> GPMSQVLFHQLVPLQVKCKDCEERRVSIRMSIELQSVSNPVHRKDLVIRLTDDTDPFFLYNLVISEEDFQSLKFQQGLLVDFLAFPQKFIDLLQQCTQEHAKEIPRFLLQLVSPAAILDNSPAFLNVVETNPEKHLTHLSLKLLPGNDVEIKKF

Centriole assembly requires oligomerization of the essential protein spindle assembly abnormal 6 (SAS-6), which forms a structural scaffold templating the organization of further organelle components. SAS-6 is an essential protein for centriole formation and a key component of a scaffold-like structure known as the “cartwheel” or “central tube”. Crystallographic, EM, atomic force microscopy, and biophysical studies of SAS-6 variants from multiple species have shown that SAS-6 oligomerization is driven by two dimerization interfaces mediated by the protein “head” domain and a homodimeric coiled-coil domain. The SAS-6 head domain also self-associates but with lower affinity (Kd of 50–100 μm in vertebrate, nematode, and algae SAS-6) and a smaller dimerization interface compared with the coiled-coil domain.

Similar to earlier assays of CeSAS-6N, we employed dimerization-impaired variants of these domains (C. reinhardtii SAS-6N (CrSAS-6N) F145E and HsSAS-6N F131E) to ensure that the hydrophobic cavity of the dimerization interface is solvent-exposed. To elucidate the location of A11 and A12 binding to HsSAS-6N, we assigned the NMR spectra of this domain and determined the crystallographic structure of HsSAS-6N F131E at 1.46 Å resolution. Comparison of the HsSAS-6N head domain structure to that of other resolved SAS-6 variants revealed that the human protein is most similar to CrSAS-6N and the Danio rerio SAS-6 head domain, with sub-0.7 Å root mean square deviation (RMSD) of Cα atom positions. In contrast, the HsSAS-6N structure diverged more strongly from that of CeSAS-6N (∼2.8 Å Cα RMSD), largely driven by repositioning of the α1 and α2 helices. We assigned the HsSAS-6N F131E NMR spectra and quantified the spectral changes upon addition of compounds on a per-residue basis, which allowed us to locate the most affected amino acids on the domain structure. Both A11 and A12 perturb amino acids surrounding the dimerization interface, whereas addition of other compounds did not produce a similar pattern. A12 binding involved fluctuating interactions of the methylpiperidine moiety with multiple residues of the HsSAS-6N dimerization cavity (Leu-76, Val-78, Phe-83, Lys-86, Phe-87, Leu-90, His-136, and Leu-137), compared with A11 where similar but tighter interactions were formed by the compound aromatic group. We observed the formation of two stable hydrogen bonds between the A12 sulfonyl group oxygen and the HsSAS-6N Leu-77 amide and between the A12 acetamide and the Gly-75 carbonyl atoms. As seen in MD simulations of HsSAS-6N with A12, the available hydrophobic interface in this orthologue is larger than originally thought on the basis of other SAS-6 structures, and this interface could be exploited by “growing” the methylpiperidine moiety, thereby gaining human SAS-6-specific enthalpic contributions to the interaction.ATP-sensitive potassium (KATP) channels, composed of four pore-lining Kir6.2 subunits and four regulatory sulfonylurea receptor 1 (SUR1) subunits, control insulin secretion in pancreatic β-cells. KATP channel opening is stimulated by PIP2 and inhibited by ATP. Mutations that increase channel opening by PIP2 reduce ATP inhibition and cause neonatal diabetes. In addition to adenine nucleotides-dependent regulation, membrane phosphoinositides participate in the gating activation of KATP channels, as they do all other eukaryotic Kir channels.

Here, we present the cryoEM structure of the KATP channel harboring the neonatal diabetes Q52R mutation (hereinafter referred to as the SUR1/Kir6.2Q52R channel) in an open conformation bound to amphipathic molecules consistent with natural C18:0/C20:4 long-chain PI(4,5)P2. At each Kir6.2-SUR1 interface, one PIP2 molecule is bound within the site that is conserved among Kir channels (referred to as the canonical site), and a second PIP2 molecule is at an adjacent site, stacked within the regulatory interface between Kir6.2 and SUR1-TMD0 (referred to as the non-canonical site). The phosphate groups are coordinated directly by Kir6.2 residues R176 and K67 while Kir6.2-W68 forms close interaction with the inositol ring, although K170, which is about 4.5 Å away and H175, which is about 5.5 Å away, are also in close proximity. Here, the PIP2 head group interacts with surrounding residues including K39 and Q57 of Kir6.2, and N131, F132, P133, and K134 of SUR1. The structure of the PIP2-bound SUR1/Kir6.2Q52R channel has an open Kir6.2 inner helix gate. Clear cryoEM density shows rotation of the Kir6.2-F168 side chains away from the pore’s center, thus causing a dilated pore size. Specifically, the sidechains of Kir6.2-K39 and R50 flip away from ATP-interacting positions, with the K39 sidechain now coordinating PIP2 at the non-canonical site; moreover, the sidechain of Kir6.2-E51 forms a salt bridge with R54 to partially occlude the ATP binding pocket. In particular, the sidechain of Kir6.2 residue 52 (Q in WT, R in the mutant) now faces SUR1-TMD0 and interacts with SUR1-W51, tethering the Kir6.2-CTD to SUR1-TMD0 in a rotated open position. The cation-π interaction observed between Kir6.2-Q52R and SUR1-W51 in the open conformation led us to hypothesize that this interaction may contribute to the gain-of-function gating effect of the Kir6.2-Q52R mutation, by stabilizing the Kir6.2-CTD in a rotated open conformation.

>[4x]MLSRKGIIPEEYVLTRLAEDPTEPRYRTRERRARFVSKKGNCNVAHKNIRERGRFLQDVFTTLVDLKWPHTLLIFTMSFLCSWLLFAMVWWLIAFAHGDLAPGEGTNVPCVTSIHSFSSAFLFSIEVQVTIGFGGRMVTEECPLAILILIVQNIVGLMINAIMLGCIFMKTAQAHRRAETLIFSKHAVITLRHGRLCFMLRVGDLRKSMIISATIHMQVVRKTTSPEGEVVPLHQVDIPMENGVGGNSIFLVAPLIIYHVIDSNSPLYDLAPSDLHHHQDLEIIVILEGVVETTGITTQARTSYLADEILWGQRFVPIVAEEDGRYSVDYSKFGNTVKVPTPLCTARQLDEDRSLLDALTLASSRGPLRKRSVAVAKAKPKFSISPDSLS;>[4x]MPLAFCGTENHSAAYRVDQGVLNNGCFVDALNVVPHVFLLFITFPILFIGWGSQSSKVHIHHSTWLHFPGHNLRWILTFILLFVLVCEIAEGILSDGVTESRHLHLYMPAGMAFMAAITSVVYYHNIETSNFPKLLIALLIYWTLAFITKTIKFVKFYDHAIGFSQLRFCLTGLLVILYGMLLLVEVNVIRVRRYIFFKTPREVKPPEDLQDLGVRFLQPFVNLLSKGTYWWMNAFIKTAHKKPIDLRAIGKLPIAMRALTNYQRLCVAFDAQARKDTQSPQGARAIWRALCHAFGRRLILSSTFRILADLLGFAGPLCIFGIVDHLGKENHVFQPKTQFLGVYFVSSQEFLGNAYVLAVLLFLALLLQRTFLQASYYVAIETGINLRGAIQTKIYNKIMHLSTSNLSMGEMTAGQICNLVAIDTNQLMWFFFLCPNLWAMPVQIIVGVILLYYILGVSALIGAAVIILLAPVQYFVATKLSQAQRSTLEHSNERLKQTNEMLRGMKLLKLYAWESIFCSRVEVTRRKEMTSLRAFAVYTSISIFMNTAIPIAAVLITFVGHVSFFKESDLSPSVAFASLSLFHILVTPLFLLSSVVRSTVKALVSVKKLSEFLSSAEIREEQCAPREPAPQGQAGKYQAVPLKVVNRKRPAREEVRDLLGPLQRLAPSMDGDADNFCVQIIGGFFTWTPDGIPTLSNITIRIPRGQLTMIVGQVGCGKSSLLLATLGEMQKVSGAVFWNSNLPDSEGEDPSSPERETAAGSDIRSRGPVAYASQKPWLLNATVEENITFESPFNKQRYKMVIEACSLQPDIDILPHGDQTQIGERGINLSGGQRQRISVARALYQQTNVVFLDDPFSALDVHLSDHLMQAGILELLRDDKRTVVLVTHKLQYLPHADWIIAMKDGTIQREGTLKDFQRSECQLFEHWKTLMNRQDQELEKETVMERKASEPSQGLPRAMSSRDGLLLDEEEEEEEAAESEEDDNLSSVLHQRAKIPWRACTKYLSSAGILLLSLLVFSQLLKHMVLVAIDYWLAKWTDSALVLSPAARNCSLSQECDLDQSVYAMVFTLLCSLGIVLCLVTSVTVEWTGLKVAKRLHRSLLNRIILAPMRFFETTPLGSILNRFSSDCNTIDQHIPSTLECLSRSTLLCVSALTVISYVTPVFLVALLPLAVVCYFIQKYFRVASRDLQQLDDTTQLPLLSHFAETVEGLTTIRAFRYEARFQQKLLEYTDSNNIASLFLTAANRWLEVRMEYIGACVVLIAAATSISNSLHRELSAGLVGLGLTYALMVSNYLNWMVRNLADMEIQLGAVKRIHALLKTEAESYEGLLAPSLIPKNWPDQGKIQIQNLSVRYDSSLKPVLKHVNALISPGQKIGICGRTGSGKSSFSLAFFRMVDMFEGRIIIDGIDIAKLPLHTLRSRLSIILQDPVLFSGTIRFNLDPEKKCSDSTLWEALEIAQLKLVVKALPGGLDAIITEGGENFSQGQRQLFCLARAFVRKTSIFIMDEATASIDMATENILQKVVMTAFADRTVVTIAHRVHTILSADLVMVLKRGAILEFDKPETLLSQKDSVFASFVRADK>[6x]GPLGSPMYVYESTVHCTNILLGLNDQRKKDILCDVTLIVERKEFRAHRAVLAACSEYFWQALVGQTKNDLVVSLPEEVTARGFGPLLQFAYTAKLLLSRENIREVIRC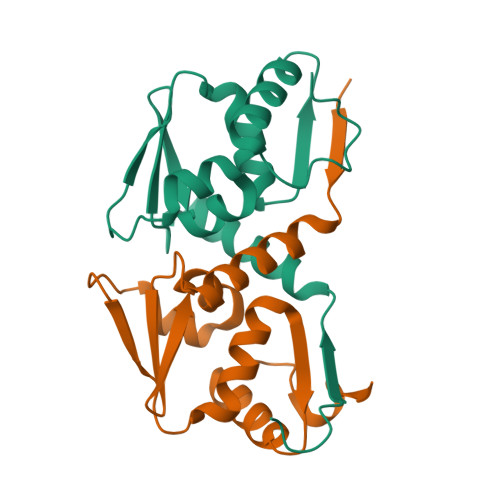AEFLRMHNLEDSCFSFL>[6x]MYYLGKELQKRSEELSRGFYELVYPPVDMYEEGGYLVVVADLAGFNKEKIKARVSGQNELIIEAEREITEPGVKYLTQRPKYVRKVIRLPYNVAKDAEISGKYENGVLTIRIPIA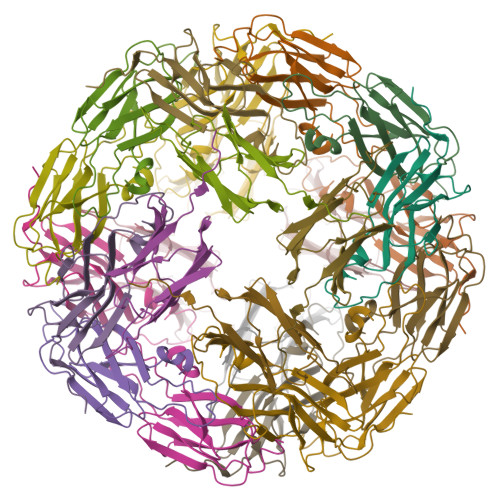GTSVIKIE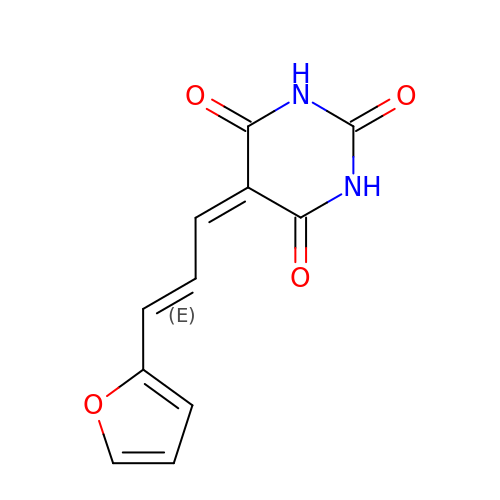5-[(E)-3-(furan-2-yl)prop-2-enylidene]-1,3-diazinane-2,4,6-trione | C11 H8 N2 O4 | PRGJOMANJQAXIH-HNQUOIGGSA-N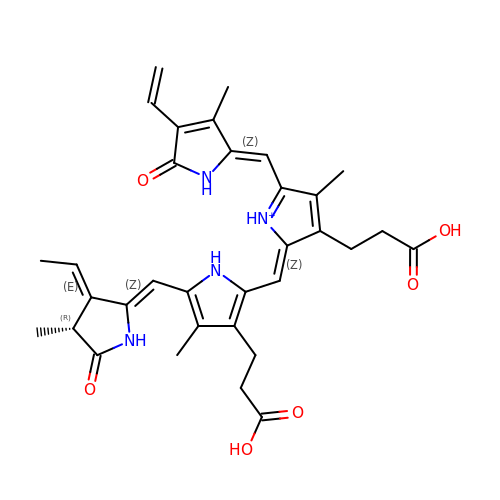3-[2-[(Z)-[5-[(Z)-(4-ethenyl-3-methyl-5-oxidanylidene-pyrrol-2-ylidene)methyl]-3-(3-hydroxy-3-oxopropyl)-4-methyl-pyrrol-1-ium-2-ylidene]methyl]-5-[(Z)-[(3E,4R)-3-ethylidene-4-methyl-5-oxidanylidene-pyrrolidin-2-ylidene]methyl]-4-methyl-1H-pyrrol-3-yl]propanoic acid | C33 H37 N4 O6 | DKMLMZVDTGOEGU-UAWLBFNISA-O>MAQIPTLREGQGKLYDFTLNGMTVTRDTVNTVVALEFLVNASPDLLSLTIGEGLSEETKFKHLLVKHAGMTRKRIEERLGRISRRVSVTVDAIIITNRKGQRFEFNRKQYLDIAKQAMKLKLPGINCVDIPTALAFLEEVLATALKDTEGSQDD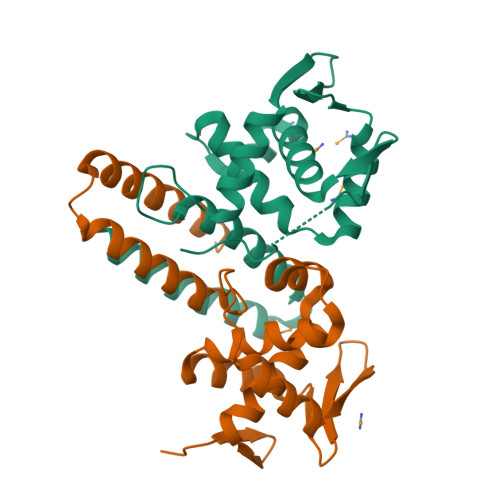RMALKADTSAAINHFREMLK[2x]>[2x]SNAMFCYQCQETVGNKGCTQVGVCGKKPETAALQDALIYVTKGLGQIATRLRAEGKAVDHRIDRLVTGNLFATITNANFDDDILAERVRMTCAAKKELAASLTDKSGLSDAALWEASEKSAMLAKAGTVGVMATTDDDVRSLRWLITFGLKGMAAYAKHADVLGKHENSLDAFMQEALAKTLDDSLSVADLVALTLETGKFGVSAMALLDAANTGTYGHPEITKVNIGVGSNPGILISGHDLRDLEMLLKQTEGTGVDVYTHSEMLPAHYYPAFKKYAHFKGNYGNAWWKQKEEFESFNGPVLLTTNCLVPPKDSYKDRVYTTGIVGFTGCKHIPGEIGEHKDFSAIIAHAKTCPAPTEIESGEIIGGFAHN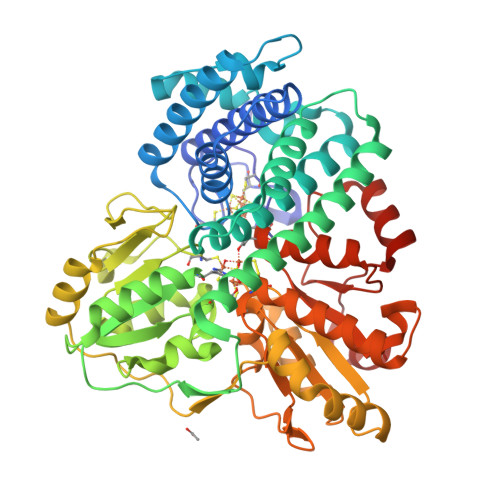QVLALADKVIDAVKSGAIKKFVVMAGCDGRAKSRSYYTDFAEGLPKDTVILTAGCAKYRYNKLNLGDIGGIPRVLDAGQCNDSYSLAVIALKLKEVFGLEDVNDLPIVYNIAWYEQKAVIVLLALLSLGVKNIHLGPTLPAFLSPNVAKVLVEQFNIGGITSPQDDLKAFFG Bacteriophage T5, a representative member of the T5-like family of siphophages, serves as an excellent model for studying the assembly, infection, cell wall perforation, and DNA ejection mechanisms of this phage family. In this study, we used cryo-electron microscopy (cryo-EM) to determine the structures of mature T5 (a laboratory-adapted, fiberless T5 mutant) and urea-treated empty T5 (lacking the tip complex) at near-atomic resolutions. The T5 head comprises 775 copies of MCP gp8, arranged into 11 pentons and 120 hexons, forming an icosahedral shell with a triangle number (T) of 13. The T5 tail, which comprises 40 trimeric rings of the TTP and a distal tip complex, is connected to a unique five-fold vertex of the head by the connector complex.

Using the local reconstruction method, we then obtained the structures of the connector complex and the portal of mature T5 at resolutions of 4.8 and 3.2 Å, respectively. The T5 portal consists of 12 copies of pb7, which replaces a penton at a unique vertex of the head and provides an entry and exit channel for DNA packaging and ejection. Based on our density map, we built an atomic model of pb7 from residues 11 to 377 of the total 403 residues. According to the domain nomenclature of the portal protein, each pb7 monomer can be divided into four domains: a crown domain (residues 337–377), a wing domain (residues 11–175, and 278–336), a stem domain (residues 176–200, and 263–277), and a clip domain (residues 201–262). Imposing C12 symmetry on the portal by means of local reconstruction revealed that the wing domain’s positively charged residue, lys77, was anchored to the DNA fragment, clearly indicating the major and minor grooves of the double-stranded DNA. We built an atomic model of adaptor protein p144 comprising all 170 residues. The adaptor is composed of 12 copies of p144, exhibiting structurally conserved conformation, as observed in many phages. Each p144 monomer contains an attachment domain (residues 46–110) and a helix bundle domain (residues 1–45 and 111–170). The attachment domain is anchored to the outer surface of the portal, whereas the helix bundle domain is attached to the top of the tail terminator. Notably, the loop (residues 14–20) of the helix bundle domain between two adjacent p144 monomers undergoes conformational changes to mediate the structural symmetry mismatch between the 12-fold symmetric adaptor and the 6-fold symmetric tail terminator p142.

>[12x]MGFKSWITEKLNPGQRIIRDMEPVSHRTNRKPFTTGQAYSKIEILNRTANMVIDSAAECSYTVGDKYNIVTYANGVKTKTLDTLLNVRPNPFMDISTFRRLVVTDLLFEGCAYIYWDGTSLYHVPAALMQVEADANKFIKKFIFNNQINYRVDEIIFIKDNSYVCGTNSQISGQSRVATVIDSLEKRSKMLNFKEKFLDNGTVIGLILETDEILNKKLRERKQEELQLDYNPSTGQSSVLILDGGMKAKPYSQISSFKDLDFKEDIEGFNKSICLAFGVPQVLLDGGNNANIRPNIELFYYMTIIPMLNKLTSSLTFFFGYKITPNTKEVAALTPDKEAEAKHLTSLVNNGIITGNEARSELNLEPLDDEQMNKIRIPANVAGSATGVSGQEGGRPKGSTEGD;>MQIITAEDYRLYGGLKRPELESGVEVMITAANALITSLLGMDDADAVDQLITTKPTRKKYFLSSPSATSVTKMTINDKEIDPEQYKLYSDGVILLKFNPPEGYMDVEYTQGGFNPMPEDLKLAACMLVDHWHKQDYRQARTIGGETVTFNNTKSGIPEHIRTIIEVYRRV[12x]> MDSFGVEGDHQADTTVLKAVFLPFISKSHLIRVVDKARIFAMHGVDVTIITTPANAAAFQTSIDHDSSRSRSIKTHIVPFPQVPGLPQGFERLDADTPQHLLPKIYQGLSILQEQFQQLFREMRPDFIVTDMYYPWSVDAAAELGIPRLVCNGGSYFAQSAVNSIELFSPQAKVDSNTETFLLPGLPHEVEMTRLQLPDWLRGAPNEYTYLMKMIKDSERKSYGSLFNSFYELEGTYEEHYKKAMGTKSWSVGPVSLWVNQDASDKACRGDVKEGKGDGVVLTWLDSKTEDSVLYVSFGSMNKFPKTQLVEIAHALEDSGHDFIWVVGKIEEGEGGADFLREFEKKVKEKNRGYLIWGW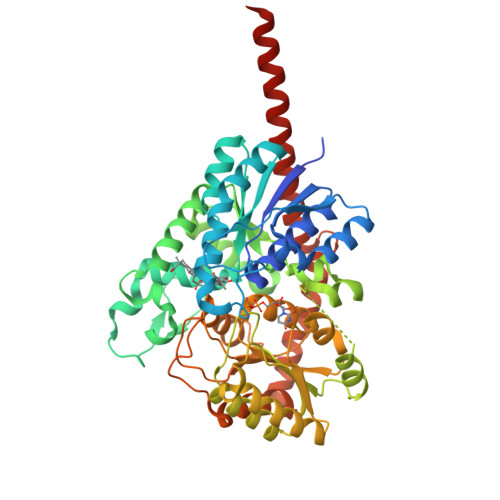APQLLILEHPAVGAVVTHCGWNTVMESVNASLPLATWPLFAEQFFNEKLVVDVVKIGVPVGVKEWRNWNEFGDEVVKREDIGKAIAFLMGGGDESLEMRKRVKVLSGATKKAIQVDGSSYTKLKELIEELKSIKLQKVNNKLMEAVALEHHHHHH>SMLTLNNIRQYYVLCEHRKDKYQALCNIYGSITIGQAIIFCQTR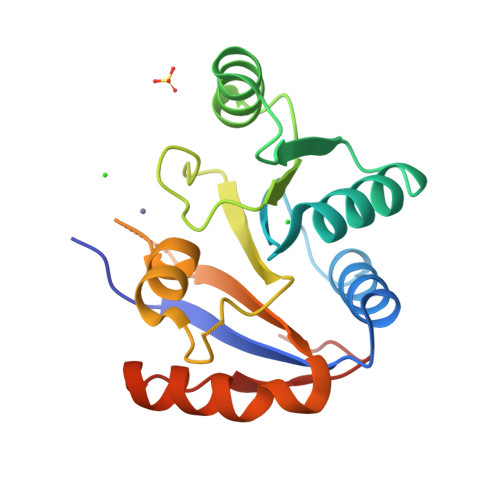RNAKWLTVEMIQDGHQVSLLSGELTVEQRASIIQRFRDGKEKVLITTNVCARGIDVKQVTIVVNFDLPVKQGEEPDYETYLHRIGRTGRFGKKGLAFNMIEVDELPSLMKIQDHFNSSIKQLNAEDMDEIE[2x]>[2x]MHHHHHHSSGRENLYFQ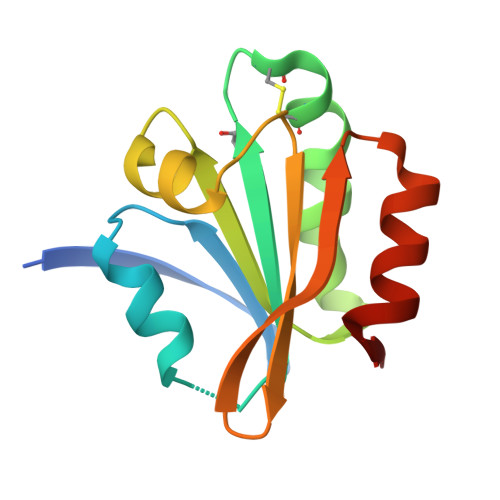GQSIYIELKNTGSLNQVFSSTQNSSIVIKFGAVWCKPCNKIKEYFKNQLNYYYVTLVDIDVDIHPKLNDQHNIKALPTFEFYFNLNNEWVLVHTVEGANQNDIEKAFQKYCLEKAK> ALSEQLKHCNGILKELLSKKHAAYAWPFYKPVDASALGLHDYHDIIKHPMDLSTVKRKMENRDYRDAQEFAADVRLMFSNCYKYNPPDHDVVAMA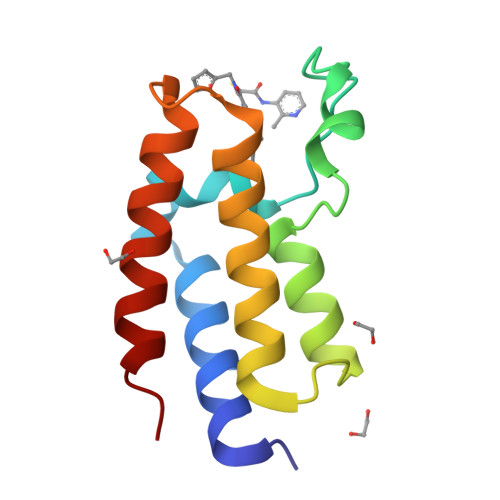RKLQDVFEFRYAKMP>GHMAPAPPANSGESSLLSESELPAGISYAEAMEGGSRPLLHPDNPVVFFDISIGSHEAGRIKIELFKNLAPKSAENFRQFCTGEFRQNQVPIGYKGATFHRIIKNFMIQGGDFVKGDGTGRLSIYGSSFPDEAFVLPHFRSGLLSLANSGPDTNGCQFFITCAKCDWLNRKHVVFGQVLGKESMQVVRKIEHVTVDGGNRPRIPVTVTQCGEL[2x];>[2x]ALLV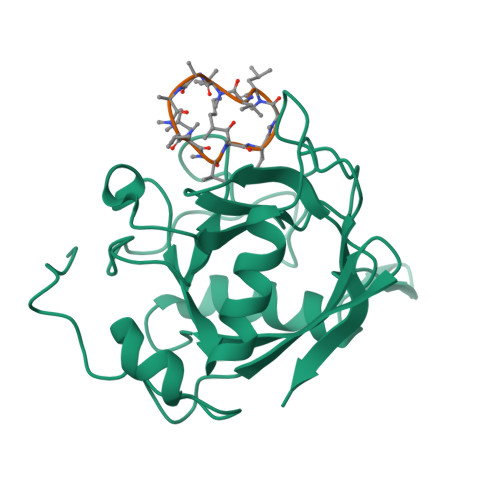TAGLVLA>[2x]MGPAFEFAVAMMKRNSSTVKTEYGEFTMLGIYDRWAVLPRHAKPGPTILMNDQEVGVLDAKELVDKDGTNLELTLLKLNRNEKFRDIRGFLAKEEVEVNEAVL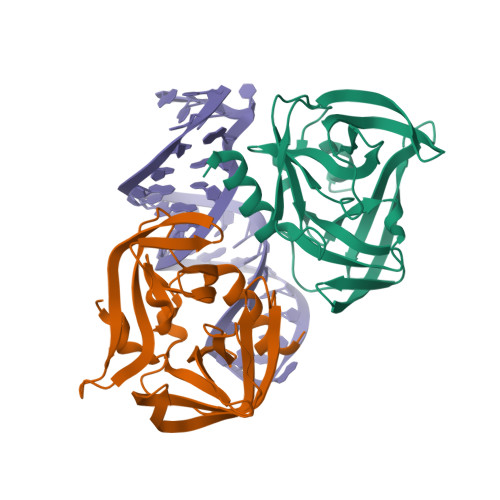AINTSKFPNMYIPVGQVTEYGFLNLGGTPTKRMLMYNFPTRAGQAGGVLMSTGKVLGIHVGGNGHQGFSAALLKHYFNDEQLEHHHHHH>[2x]MMMKRDYGGVGTIALRASALLKAMSQDIEDQRKEFNQTEYYQTFTRNAVAKLPKLSRRIVDQAIKEMEEDGYQFNKKQVGNVEQYALTIQNVIDIYAHRKIPKYRD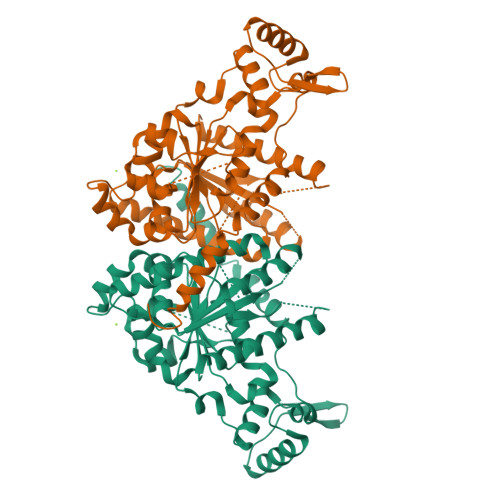IHKSPYVIFVVNLKGGVSKTVSTVTLAHALRVHQDLLRHDLRILVIDLDPQASSTMFLDHTHSIGSILETAAQAMLNNLDAETLRKEVIRPTIVPGVDVIPASIDDGFVASQWRELVEEHLPGQNQYEILRRNIIDRVADDYDFIFIDTGPHLDPFLLNGLAASDLLLTPTPPAQVDFHSTLKYLTRLPEMLEQLEEEGVEPRLSASIGFMSKMTGKRDHETSHSLAREVYASNILDSSLPRLDGFERCGESFDTVISANPQSYPGSAEALKKARTEAERFTKAVFDRIEFVRGEAA>MAEELVLERCDLELETNGRDHHTADLCREKLVVRRGQPFWLTLHFEGRNYEASVDSLTFSVVTGPAPSQEAGTKARFPLRDAVEEGDWTATVVDQQDCTLSLQLTTPANAPIGLYRLSLEASTGYQGSSFVLGHFILLFNAWCPADAVYLDSEEERQEYVLTQQGFIYQGSAKFIKNIPWNFGQFEDGILDICLILLDVNPKFLKNAGRDCSRRSSPVYVGRVVSGMVNCNDDQGVLLGRWDNNYGDGVSPMSWIGSVDILRRWKNHGCQRVKYGQCWVFAAVACTVLRCLGIPTRVVTNYNSAHDQNSNLLIEYFRNEFGEIQGDKSEMIWNFHCWVESWMTRPDLQPGYEGWQALDPTPQEKSEGTYCCGPVPVRAIKEGDLSTKYDAPFVFAEVNADVVDWIQQDDGSVHKSINRSLIVGLKISTKSVGRDEREDITHTYKYPEGSSEEREAFTRANHLNKLAEKEETGMAMRIRVGQSMNMGSDFDVFAHITNNTAEEYVCRLLLCARTVSYNGILGPECGTKYLLNLNLEPFSEKSVPLCILYEKYRDCLTESNLIKVRALLVEPVINSYLLAERDLYLENPEIKIRILGEPKQKRKLVAEVSLQNPLPVALEGCTFTVEGAGLTEEQKTVEIPDPVEAGEEVKVRMDLLPLHMGLHKLVVNFESDKLKAVKGFRNVIIGPALEHHHHHH[3x]

Transglutaminase 2 (TG2) is a multi-functional protein that possesses various biological activities, including protein cross-linking activity, GTPase activity, protein disulfide isomerase activity, kinase activity, and scaffold activity. Human TG2 is 687 amino acids in length, consisting of four domains, an N-terminal β-sandwich domain, catalytic domain, and two C-terminal β-barrel domains, and is the most ubiquitous isoform of the TG family. When it is secreted into the extracellular environment, TG2 functions as a cross-linking enzyme in the matrix. This protein transamidase activity of TG2 is positively regulated by calcium and negatively regulated by GTP. Structural studies showed that TG2 undergoes an extraordinarily large conformational change upon activation; closed inactive form and opened active form.

Human exon sequencing data in the various sequence databases, including NCBI, Ensembl, and ESP, showed a valine residue at position 224 of TG2, supporting the idea that the G224V form, rather than the G224 form, is the natural TG2 variant. The 2.5 Å crystal structure of TG2 (G224V) was solved and refined to an Rwork of 23.6% and an Rfree of 25.6%. There were three monomers in the asymmetric unit, chain A, chain B, and chain C. All three chains were identical and contained GTP, which is similar to that of the recently solved GTP-bound form of TG2 (G224). The root mean square deviations (RMSD) between the TG2 (G224) and TG2 (G224V) variants was 0.51 Å, indicating that replacement of G224 with valine did not have any effect on the overall structure of TG2. The G224 site on the structure was carefully analyzed and we found that the amino acid residue at site 224 is a critical residue for the formation of hydrophobic clusters with neighboring hydrophobic residues, including V287 and L288, which are located on active site cysteine (C277)-containing ɑ-helix in the catalytic core. The active site cysteine (C277)-containing ɑ-helix, which is stabilized by the formation of a hydrophobic cluster with neighboring V224, was shifted to the opposite direction by 16°, especially the active site cysteine region. Moreover, TG2 (G224V) was approximately 4.4-fold more sensitive to Ca2+ than TG2 (G224), with Ca2+ EC50 values of 0.211±0.038 mM and 0.929±0.06 mM, respectively. Stability analysis of the two forms showed that TG2 gains stability by mutating glycine to valine at position 224. Based on these results, we conclude that hydrophobic patch formation, via the newly introduced G224V, may lead to fixation between G224-containing α-helix, which is connected to the Ca2+-binding site loop, and active site cysteine (C277)-containing α-helix.> GVLPVEKCNLEDSACMTSAFQQALPTFVAGLPDHGVEVMDVLDLDDFAFDLSGLQFTLKEGKLKGLKGAVIDNVKWDLKKKNIEVDFHLDATVKGHYTAGGRILILPITGDGQMKLKLKNIHIHLVVSYEMEKDAEGVDHVIFKKYTVTFDVKDNAQFGLTNLFNGNKELSDTMLTFLNQNWKQVSEEFGKPVME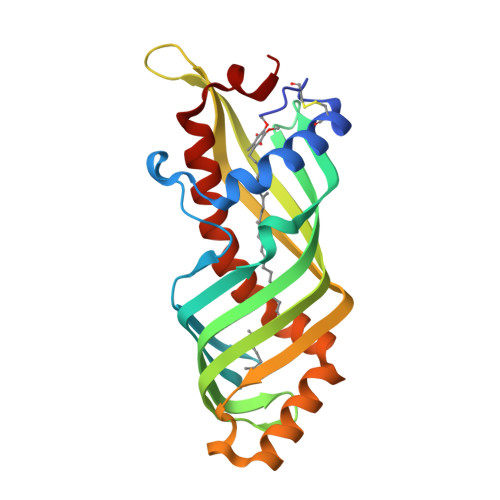AAAKKIFKNIKHFLAKVPIAEIANV>MALADISGYLDVLDSVRGFSYLENAREVLRSGEARCLGNPRSEPEYVKALYVIGASRIPVGDGCSHTLEELGVFDISVPGEMVFPSPLDFFERGKPTPLVRSRLQLPNGVRVWLKLEWYNPFSLSVADRPAVEIISRLSRRVEKGSLVADATSSNFGVALSAVARLYGYRARVYLPGAAEEFGKLLPRLLGAQVI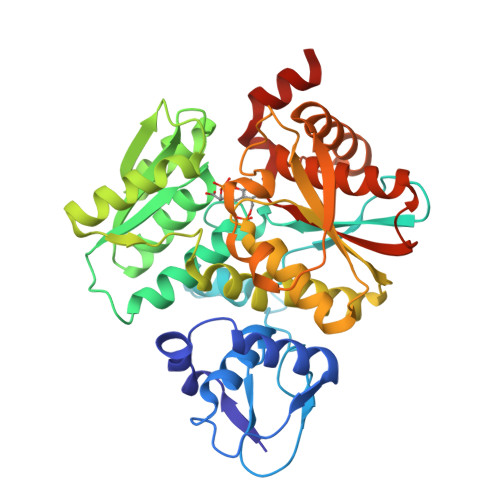VDPEAPSTVHLLPRVMKDSKNEGFVHVNQYYNDANFEAHMRGTAREIFVQSRRGGLALRGVAGSLGTSGHMSAAAFYLQSVDPSIRAVLVQPAQGDSIPGIRRVETGMLWINMLDISYTLAEVTLEEAMEAVVEVARSDGLVIGPSGGAAVKALAKKAAEGDLEPGDYVVVVPDTGFKYLSLVQNALEGAGDSV[4x]Three human ‘MBL-fold’ DNA repair factors, SNM1A, SNM1B (Apollo) and SNM1C (Artemis) are involved in repair of ICLs and DSBs. SNM1A–C have conserved β-CASP and metallo-β-lactamase (MBL) domains. SNM1A/SNM1B are 5′–3′ exonucleases with the unusual capacity to hydrolyse DNA substrates containing lesions, including ICLs. SNM1A has a role in replication-coupled ICL repair, functioning with the endonuclease, XPF-ERCC1, to effectively “unhook” the ICL and allow downstream processing.

Interestingly introduction of an extra carbonyl group at position 2′ (as in amide 20), resulted in a 100-fold decrease in potency when compared to 13, while against SNM1B and SNM1C inhibitors 13 and 20 show inhibition with a similar range. As was the case for the initial ELF hit compound soaking, crystals were back-soaked to remove malonate ions with or without 500 μM ZnCl2 to obtain the mono- and di-metal forms suitable for soaking different classes of inhibitors. We obtained structures for SNM1A complexed with three derivatives of 6 (13, 20, and 19) at resolutions ranging from 1.5 to 1.8 Å (Fig. 5A and ESI 9†). All of these compounds bind to SNM1A with very similar orientations. Their quinazoline ring is positioned to stack with D736, in an equivalent position to the adenine moiety in the SNM1B nucleotide complex. The hydroxamate group binds to both metal ions with its carbonyl oxygen coordinating with M1 and with its hydroxyl group bridging M1 and M2, the latter likely in a manner similar to the nucleophilic water. A hydrogen bond is formed between one of the carboxylate oxygens and D736 and the nitrogen of the hydroxamate moiety with all three compounds. The R1 methyl group of the inhibitors is directed towards the side chains of H734 and S880. The binding modes of the R2 substituents are more diverse, but all of them occupy a similar position close to K883, Y841 and G963. These three residues form the binding pocket of the 5′ phosphate of the substrate, which has been shown to be a key determinant of DNA binding and exonuclease activity for SNM1B.26 With all three inhibitors, the R2 groups are positioned in an equivalent position to the ribose ring of the nucleotide in the SNM1B nucleotide complex, but do not extend into the phosphate binding pocket itself.

> KKTCPFYKKIPGTGFTVDAFQYGVVEGCTAYFLTHFHSDHYAGLSKHFTFPVYCSEITGNLLKNKLHVQEQYIHPLPLDTECIVNGVKVVLLDANHCPGAVMILFYLPNGTVILHTGDFRADPSMERSLLADQKVHMLYLDTTYCSPEYTFPSQQEVIRFAINTAFEAVTLNPHALVVCGTYSIGKEKVFLAIADVLGSKVGMSQEKYKTLQCLNIPEINSLITTDMCSSLVHLLPMMQINFKGLQSHLKKCGGKYNQILAFRPTGWTHSNKFTRIADVIPQTKGNISIYGIPYSEHSSYLEMKRFVQWLKPQKIIPTVNVGTWKSRSTMEKYFREWKLEAGY>[2x]GSHMAPLKDVYKNDFLIGNAISAE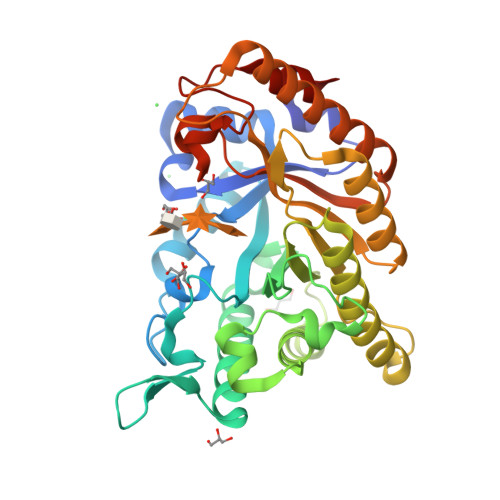DLEGTRLELLKMHHDVVTAGNAMKPDALQPTKGNFTFTAADAMIDKVLAEGMKMHGHVLVWHQQSPAWLNTKKDDNNNTVPLGRDEALDNLRTHIQTVMKHFGNKVISWDVVNEAMNDNPSNPADYKASLRQTPWYQAIGSDYVEQAFLAAREVLDENPSWNIKLYYNDYNEDNQNKATAIYNMVKDINDRYAAAHNGKLLIDGVGMQGHYNINTNPDNVKLSLEKFISLGVEVSVSELDVTAGNNYTLPENLAVGQAYLYAQLFKLYKEHADHIARVTFWGMDDNTSWRAENNPLLFDKNLQAKPAYYGVIDPAEQ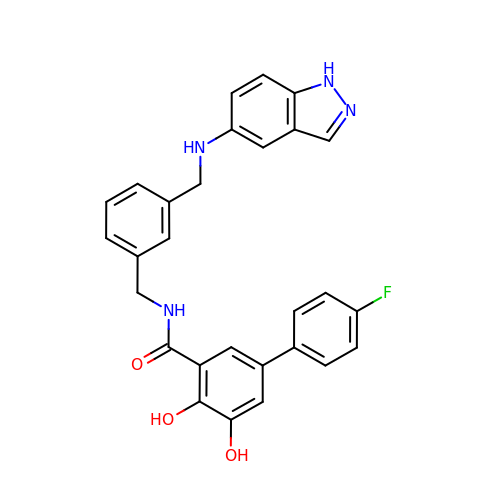5-(4-fluorophenyl)-2,3-dihydroxy-N-[[3-[(1H-indazol-5-ylamino)methyl]phenyl]methyl]benzamide | C28 H23 F N4 O3 | XPYHTFSFVXFLFG-UHFFFAOYSA-N>MSNATLNQLPGRLGDPSMSLGTDPRTDPRLAAALTQLGLADQAAEPPVNANSEVADCIAYSTAAEQAWQTLGAMLGSQGEPSNPVDVREETIKGRGGNEIKLYIHSPTGHTSDSDPLPCVVHTHGGGMVILTAADANYSRWRSELAATGLVVVGVEFRNAAGALGNHPFPAGLHDCADAAKWVASNREALGISTLIMSGESGGGNLSLATTMLAKKEGWLEEIAGVYAQCPYISGLYASKPEELPSLLENDAYFLDMKTMGAM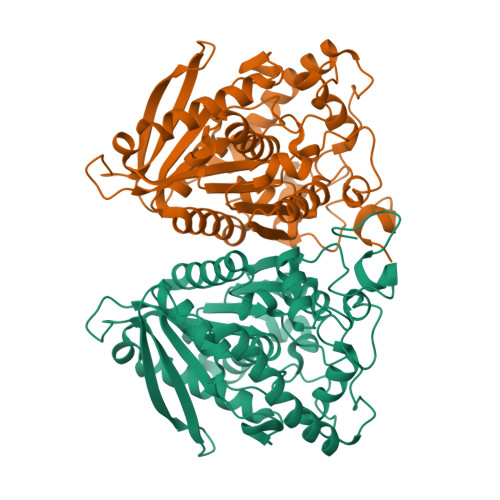VKPYDPTGENASNPLAWPYHASLEDLAGLPPHVISVNELDPLRDEGLAHYRKLLKAGVSTVGRTVHGTCHAADCSFVDVIPDVYFATVRDISAFAYSRA[4x]>MRKEAIYHRPADNFAYAYDSETLHLRLRTKKDDIDRVELLHGDPYDWQNGAWQFQMMPMRKTGSDELFDYWFAEVKPPYRRLRYGFVLYSGEEKLVYTEKGFYFEVPTDDTAYYFCFPFLHRVDLFEAPDWVKDTVWYQIFPERFANGNPSISPEGSRPWGSEDPTPTSFFGGDLQGIIDHLDYLVDLGITGIYLTPIFRSPSNHKYDTADYFEVDPHFGDKETLKTLIDRCHEKGIRVMLDAVFNHCGYEFAPFQDVWKNGESSKYKDWFHIHEFPLQTEPRPNYDTFAFVPQMPKLNTANPEVKRYLLDVATYWIREFDIDGWRLDVANEIDHEFWREFRQEVKALKPDVYILGQIWHDAMPWLRGDQFDAVMNYPFTDGVLRFFAKEEISARQFANQMMHVLHSYPNNVNEAAFNLLGSHDTSRILTVCGGDIRKVKLLFLFQLTFTGSPCIYYGDEIGMTGGNDPECRKCMVWDPMQQNKELHQHVKQLIALRKQYRSLRRGEISFLHADDEMNYLIYKKTDGDETVLV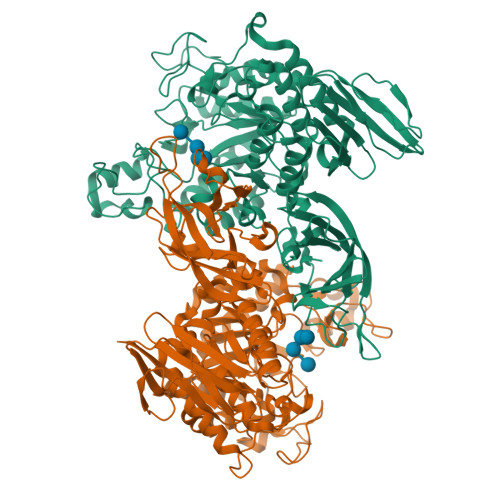IINRSDQKADIPIPLDARGTWLVNLLTGERFAAEAETLCTSLPPYGFVLYAIEHW[2x]> MCGRFAQSQTREDYLALLA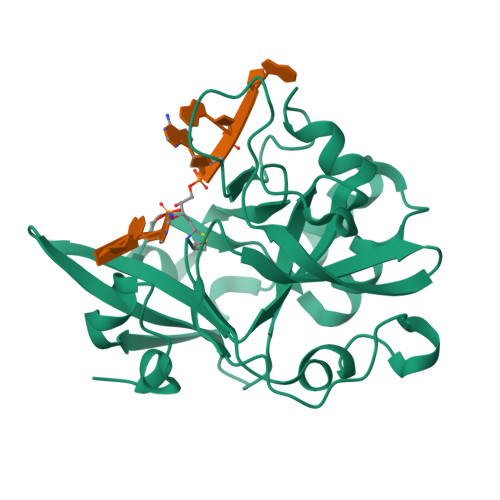EDIERDIPYDPEPIGRYNVAPGTKVLLLSERDEHLHLDPVFWGYAPGWWDKPPLINARVETAATSRMFKPLWQHGRAICFADGWFEWKKEGDKKQPFFIYRADGQPIFMAAIGSTPFERGDEAEGFLIVTAAADQGLVDIHDRRPLVLSPEAAREWMRQEISGKEASEIAASGCVPANQFSWHPVSRAVGNVKNQGAELIQPVLEVLFQ4-[(2-azanyl-1,3-benzothiazol-6-yl)oxymethyl]benzenecarbonitrile | C15 H11 N3 O S | 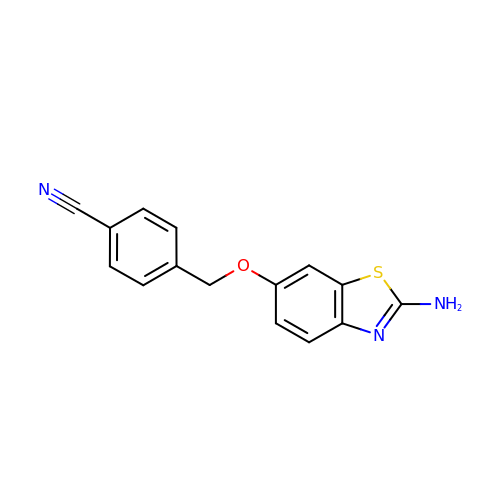ZIROAUYIWZSHKG-UHFFFAOYSA-N>GMSSVSLQDFDAERIGLFHEDIKRKFDELKSKNLKLDLTRGKPSSEQLDFADELLALPGKGDFKAADGTDVRNYGGLDGIVDIRQIWADLLGVPVEQVLAGDASSLNIMFDVISWSYIFGNNDSVQPWSKEETVKWICPVPGYDRHFSITERFGFEMISVPMNEDGPDMDAVEELVKNPQVKGMWVVPVFSNPTGFTVTEDVAKRLSAMETAAPDFRVVWDNAYAVHTLTDEFPEVIDIVGLGEAAGNPNRFWAFTSTSKITLAGAGVSFFLTSAENRKWYTGHAGIRGIGPNKVNQLAHARYFGDAEGVRAVMRKHAASLAPKFNKVLEILDSRLAEYGVAQWTVPAGGYFISLDVVPGTASRVAELAKEAGIALTGAGSSYPLRQDPENKNLRLAPSLPPVEELEVAM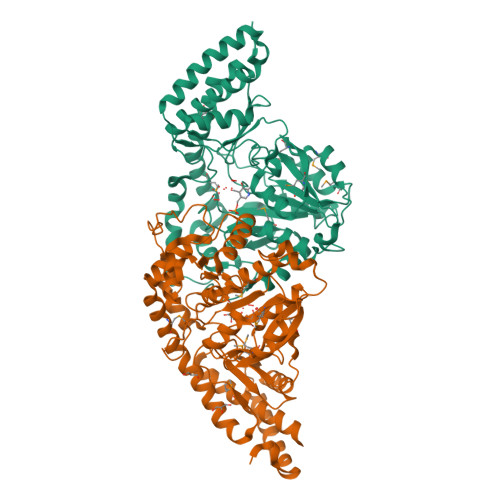DGVATCVLLAAAEHYAN[2x]>CCCGGG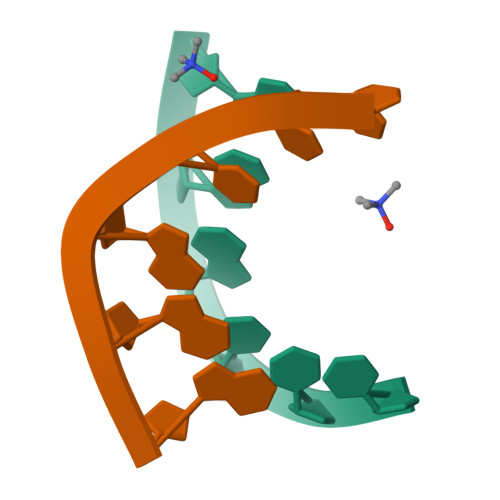[4x]> MDRAPVTTGPLDMPIMHDSDRYDFVKDIGSGNFGVARLMRDKLTKELVAVKYIERGAAIDENVQREIINHRSLRHPNIVRFKEVILTPTHLAIIMEYASGGELYERICNAGRFSEDEARFFFQQLLSGVSYCHSMQICHRDLKLENTLLDGSPAPRLKICDFGYSKSSVLHSQP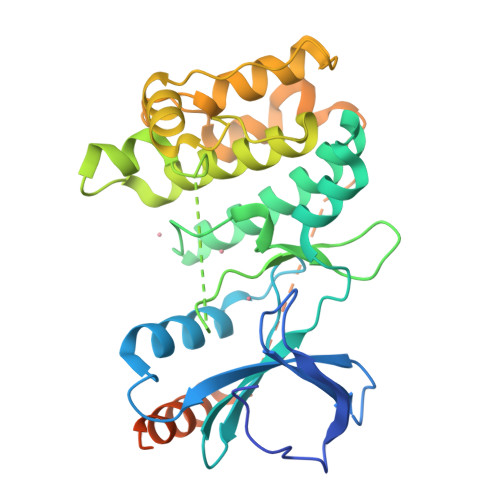KSTVGTPAYIAPEVLLRQEYDGKIADVWSCGVTLYVMLVGAYPFEDPEEPRDYRKTIQRILSVKYSIPDDIRISPECCHLISRIFVADPATRISIPEIKTHSWFLKNLPADLMNESNTGSQFQEPEQPMQSLDTIMQIISEATIPAVRNRCLDDFMTDNLDLDDDMDDFDSESEIDIDSSGEIVYAL> MRNLDFIDSFIPTEGKYIRVMDFYNSEYPFCIHAPSAPNGDIMTEICSRENNQYFIFFPTDDGRVIIANRHNGSVFTGEATSVVSDIYTGSPLQFFREVKRTMATYYLAIQNPESATDVRALEPHSHELPSRLYYTNNIENNSNILISNKEQIYLTLPSLPENEQYPKTPVLSGIDDIGPNQSEKSIIGSTLIPCIMVSDFISLGERMKTTPYYYVKHTQYWQSMWSALFPPGSKETKTEKSGITDTSQISMTDGINVSIGADFGLRFGNKTFGIKGGFTYDTKTQITNTSQLLIETTYTREYTNTENFPVRYTGYVLASEFTLHRSDGTQVNTIPWVALNDNYTTIARYPHFASEPLLGNTKIIT;> MCDSKDNSGVSEKCGKKFTNYPLNTTPTSLNYNLPEISKKFYNLKNKYSRNGYGLSKTEFPSSIENCPSNEYSIMYDNKDPRFLIRFLLDDGRYIIADRDDGEVFDEAPTYLDNNNHPIISRHYTGEERQKFEQVGSGDYITGEQFFQFYTQNKTRVLSNCRALDSRTILLSTAKIFPIYPPASETQLTAFVNSSFYAAAIPQLPQTSLLENIPEPTSLDDSGVLPKDAVRAVKGSALLPCIIVHDPNLNNSDKMKFNTYYLLEYKEYWHQLWSQIIPAHQTVKIQERTGISEVVQNSMIEDLNMYIGADFGMLFYFRSSGFKEQITRGLNRPLSQTTTQLGERVEEMEYYNSNDLDVRYVKYALAREFTLKRVNGEIVKN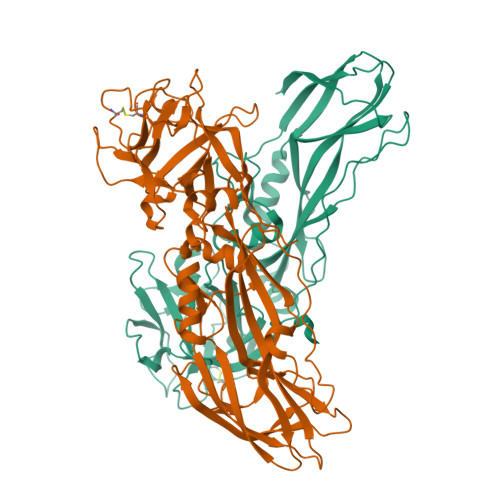WVAVDYRLAGIQSYPNAPITNPLTLTKHTIIRCENSYDGHIFKTPLIFKNGEVIVKTNEELIPKINQ>[2x]MFKTEFEFPEELKTKLQEHINYFPKKRQAILLCLHEIQNYYGYIPPESLKPLADMLELPLNHVEGVVAFYDMFDREDKAKYRIRVCVSIVCHLMGTNKLLKALENILGIKPGEVTPDGKFKIVPVQCLDACSEAPVFMVNDDEYKFESEVQLNEILSRYT;>[2x]MRSYPAIPRIYAETTLNMLLKRAKKPRVHSIDEYLKDGGYQALEKALNMSPEEIIDWVDKSTLRGRGGAGFPTGKKWKFAVQNPGPRYFICNADESEPGTFKDRIIIERDPHLLIEGIIISSYAIGANEAYIYIRGEYPAGYYILRDAIEEAKKKGFLGKNILGSGFDLEIYVARGAGAYICGEETALIESLEGKRGHPRLKPPYPVQKGLWGKPTVVNNVETIANVPFIISMGWEEYRYIGPSDYAGPKLFPVSGKVKKPGVYELPMNTTLREVIFKYAGGTLGNKKVKAVFSGALDCFSSEELDIPMDYSPLGFGGTGTVIVLTEEDDIVEAALKIAEFYEHETCGQCTPCRVGCYEQANLLEKIYKGEATEQDWEGFDFVNRNIQPTSICGLGAVAGRLIRQTLEKFPEEWEKYRKKSASLPLAGHHHHHH

Complex I couples the transfer of two electrons from NADH to ubiquinone (Q) with the translocation of four protons across the membrane. The L-shaped complex is structured into a peripheral arm that protrudes into the aqueous milieu and catalyzes electron transfer with one FMN and 8–10 iron–sulfur ([Fe–S]) clusters, and a membrane arm embedded in the lipid bilayer that mediates proton translocation. We have determined structures of the electron-input module of complex I from the hyperthermophilic bacterium Aquifex aeolicus, encompassing subunits NuoE and NuoF that contain the FMN cofactor, the [4Fe–4S] cluster N3, and the [2Fe–2S] cluster N1a, respectively, both in the air-oxidized and dithionite-reduced states at resolutions up to 1.8 Å. Here, we show that the redox state of N1a regulates NADH oxidation in complex I by inducing a conformational change close to the NADH-binding site.

We therefore sought to lock the peptide bond in place by exchanging a nearby residue, G129E, with serine and aspartate, respectively. The longer side chains were intended to occupy the position of the bound water molecule that has to make way for the flipping peptide bond according to our structures. Structures of the oxidized G129SE and G129DE variants were refined to 2.4 and 1.9 Å resolution, respectively. Overall, there were no significant changes from the original NuoEF, with the notable exception of the peptide bond of E95F that pointed away from FMN in the oxidized state of both variants, as was the case only in the reduced structures of the original protein. The same position of the peptide bond was retained when the oxidized G129DE variant was soaked with NAD+. However, no electron density for the nicotinamide ring and its ribose is detected, while the ADP moiety is well defined. Thus, the nicotinamide might adopt several positions within the binding pocket of the variant. The 3.5 Å distance between Oγ of S129E and the carbonyl oxygen of E95F is longer than the 3.2 Å from the carboxylate oxygen of D129E to this position. Thus, while both mutations fixed the position of the peptide bond, the Gly/Asp exchange seemed to exert a much stronger effect than the Gly/Ser mutation.>SEPLVRFKRSVNITKGDLNSWRTGTDPCNGKWFGIYCQKGQTVSGIHVTRLGLSGTINIEDLKDLPNLRTIRLDNNLLSGPLPPFFKLPGLKSLLLSNNSFSGEIADDFFKETPQLKRVFLDNNRLSGKIPASLMQLAGLEELHMQGNQFTGEIPPLTDGNKVLKSLDLSNNDLEGEIPITISDRKNLEMKFEGNQRLCGSPLNIECD[2x]

Plant receptor-like kinases (RLKs) play key roles in various biological processes involving plant immune defense and development. PRK3 is a type I transmembrane receptor which contains an N-terminal signal peptide domain (SP), an LRR capping domain (CD), a leucine rich repeat domain (LRR), an LRR C-terminal domain (CT), a transmembrane domain (TM), and an intracellular kinase domain (KD). In Arabidopsis thaliana, AtPRK3, along with AtPRK1, AtPRK6, and AtPRK8, have been predicted as the receptors that sense the AtLURE1.2 peptide. It has been revealed that the AtPRK3 has a vital role in pollen tube growth, plant fertility, and plant reproduction. Here we present the atomic structure of the extracellular domain (ecd) of the PRK3 (residues 20–237) from Arabidopsis thaliana resolved at 2.5 Å.

To gain a better understanding of PRK3-mediated pollen tube development, we have crystallized a protein fragment of PRK3 spanning residues 20–237 in space group P42 with two PRK3 protein molecules in each asymmetric unit. The AtPRK3 ectodomain contains six copies of plant specific LRR repeats ranging from 23–25 amino acid residues. The ectodomain forms a single continuous structure in an arc shaped conformation. There are two pairs of cysteine residues, C53 and C62, C224 and C232; they form two disulfide bonds in the CD and the CT, respectively. Two N-glycosylation sites are identified on residues N37 and N123, with only one visible GlcNAc sugar residue conjugated on N37 and two such residues on N123. We believe that the exposed N123 glycosylation pattern on the concave side of the PRK3 ectodomain can form hydrated branches and are likely to facilitate the association with other molecules. There is a positively charged electrostatic patch on the concave surface of the LRR domain, whereas the C terminal region is mostly negatively charged. Therefore, we can safely suggest that the positively charged surface will provide a favorable interacting surface for negatively charged proteins. Our size-exclusion chromatographic analysis of the recombinant PRK3 protein further supports the hypothesis that ecdPRK3 remains a monomer in solution. The PRK3 ectodomain contains six LRRs whereas SERK family members have five LRRs in their ectodomain.> GHR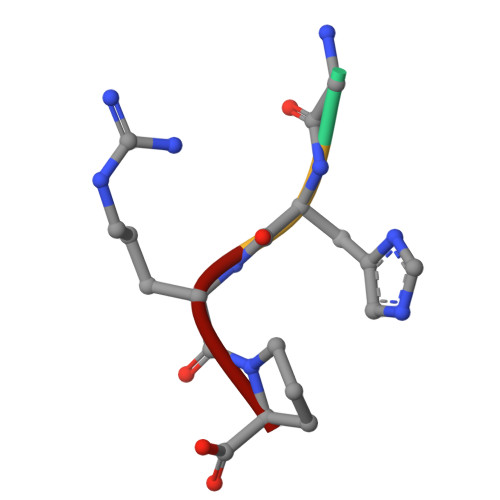P7-(diethylamino)-N-[(2S)-2-(2,4-difluorophenyl)-2-hydroxy-3-(1H-1,2,4-triazol-1-yl)propyl]-2-oxo-2H-1-benzopyran-3-carboxamide 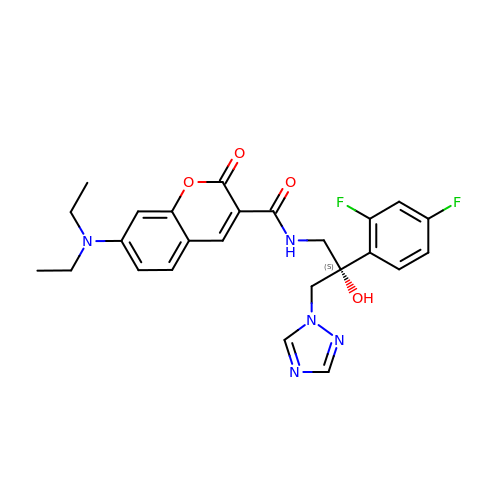| C25 H25 F2 N5 O4 | QYBYHULZZSKXIJ-VWLOTQADSA-N>[2x]MESKAKTTVTFHSGILTIGGTVIEVAYKDAHIFFDFGTEFRPELDLPDDHIETLINNRLVPELKDLYDPRLGYEYHGAEDKDYQHTAVFLSHAHLDHSRMINYLDPAVPLYTLKETKMILNSLN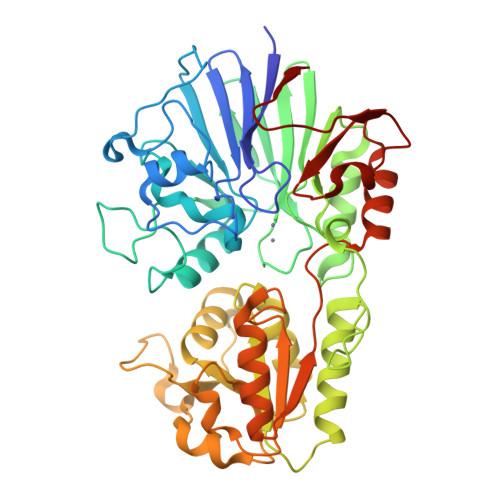RKGDFLIPSPFEEKNFTREMIGLNKNDVIKVGEISVEIVPVDHDAYGASALLIRTPDHFITYTGDLRLHGHNREETLAFCEKAKHTELLMMEGVSISFPEREPDPAQIAVVSEEDLVQHLVRLELENPNRQITFNGYPANVERFAKIIEKSPRTVVLEANMAALLLEVFGIEVRYYYAESGKIPELNPALEIPYDTLLKDKTDYLWQVVNQFDNLQEGSLYIHSDAQPLGDFDPQYRVFLDLLAKKDITFVRLACSGHAIPEDLDKIIALIEPQVLVPIHTLKPEKLENPYGERILPERGEQIVL> MLKFMLDTNICIFTIKNKPASVRERFNLNQGKMCISSVTLMELIYGAEKSQMPERNLAVIEGFVSRIDVLDYDAAAATHT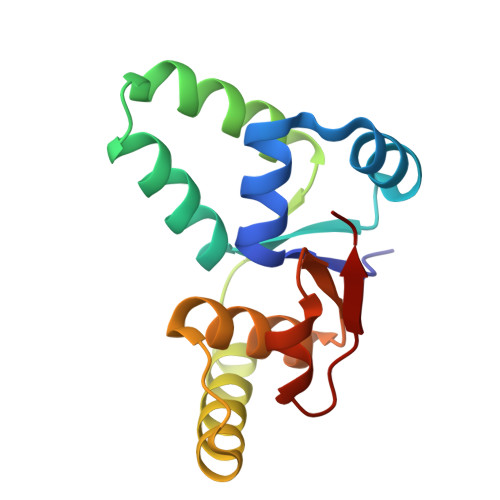GQIRAELARQGRPVGPFDQMIAGHARSRGLIIVTNNTREFERVGGLRTEDWS>DDSFPIAGIYDTTTDNKCSIKTAVAKNMLDPITGQKLLEAQAATGGIVDLLSRERYSVHKAMERGLIENTSTQRLLNAQKAFTGIEDPVTKKRLSVGEAVQKGWMPRESVLPHLQVQHLTGGLIDP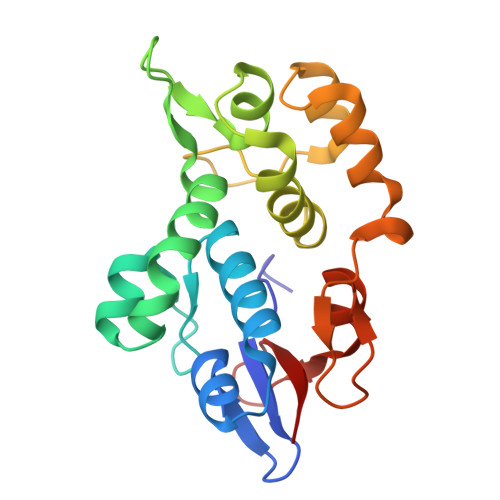KRTGRIPIQQALLSGMISEELAQLLQDESSYEKDLTDPISKERLSYKEAMGRCRKDPLSGLLLLPAA[2x]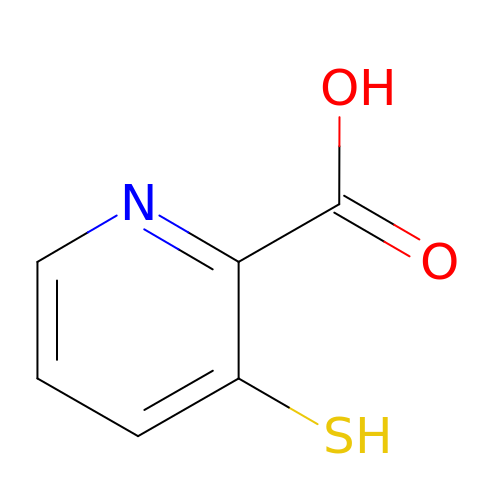3-sulfanylpyridine-2-carboxylic acid | C6 H5 N O2 S | ZYFDNIOIEFZULT-UHFFFAOYSA-N> CNIKNGRCEQFCKNSADNKVVCSCTEGYRLAENQKSCEPAVPFPCGRVSVSQTSKLTR;> VVGGEDAKPGQFPWQVVLNGKVDAFCGGSIVNEKWIVTAAHCVETGVKITVVAGEHNIEETEHTEQKRNVIRIIPHHNYNAAINT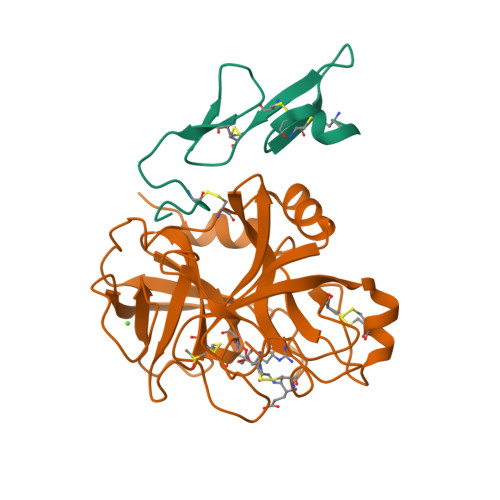YNHDIALLELDEPLVLNSYVTPICIADKEYTNIFLKFGSGYVSGWGRVFHKGRSALVLQYLRVPLVDRATCLRSTKFTIYNNMFCAGFHEGGRDSCQGDSGGPHVTEVEGTSFLTGIISWGEECAMKGKYGIYTKVSRYVNWIKEKTKLT>[2x]MRGSPHHHHHHGSAKNVVLDHDGNLDDFVAMVLLASNTEKVRLIGALCTDADCFVENGFNVTGKIMCLMHNNMNLP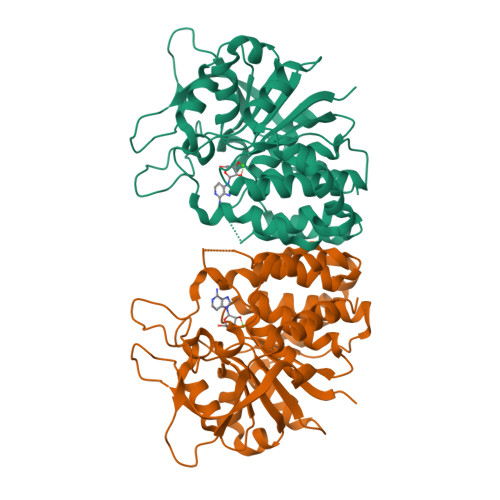LFPIGKSAATAVNPFPKEWRCLAKNMDDMPILNIPENVELWDKIKAENEKYEGQQLLADLVMNSEEKVTICVTGPLSNVAWCIDKYGEKFTSKVEECVIMGGAVDVRGNVFLPSTDGTAEWNIYWDPASAKTVFGCPGLRRIMFSLDSTNTVPVRSPYVQRFGEQTNFLLSILVGTMWAMCTHCELLRDGDGYYAWDALTAAYVVDQKVANVDPVPIDVVVDKQPNEGATVRTDAENYPLTFVARNPEAEFFLDMLLRSARAC> GAMD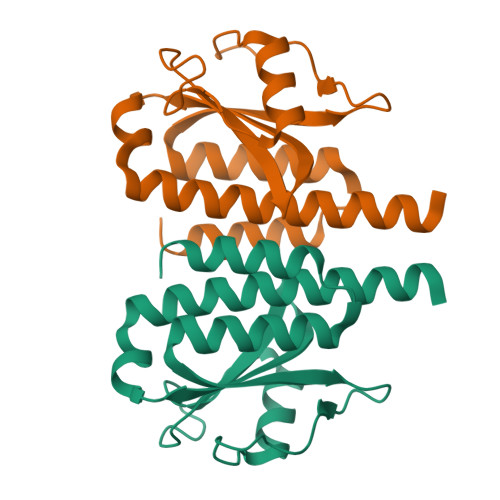LYEMSKALAVGRSPQDIAATSEQFIASTFHARSQVLLPDDNGKLQPLTHPQGMTPWDDAIAQWSFDKGLPAGAGTDTLPGVPYQILPLKSGEKTYGLVVVEPGNLRQLMIPEQQRLLETFTLLVANALERLTKLAAALEHHHHHH>MQEVQSSRSGRGGNFGFGDSRGGGGNFGPGPGSNFRGGSDGYGSGRG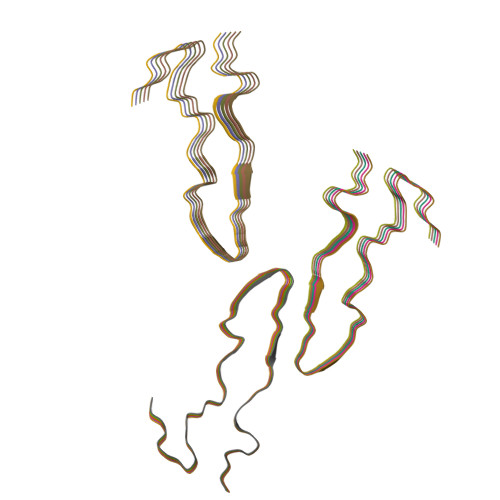FGDGYNGYGGGPGGGNFGGSPGYGGGRGGYGGGGPGYGNQGGGYGGGYDNYGGGNYGSGNYNVFGNYNQQPSNYGPMKSGNFGGSRNMGGPYGGGNYGPGGSGGSGGYGGRSRY[15x]> MTQAKAKHADVPVNLYRPNAPFIGKVISNEPLVKEGGIGIVQHIKFDLTGGNLKYIEGQSIGIIPPGVDKNGKPEKLRLYSIASTRHGDDVDDKTISLCVRQLEYKHPESGETVYGVCSTYLTHIEPGSEVKITGPVGKEMLLPDDPEANVIMLATGTGIAPMRTYLWRMFKDAERAANPEYQFKGFSWLVFGVPTTPNILYKEELEEIQQKYPDNFRLTYAISREQKNPQGGRMYIQDRVAEHADQLWQLIKNQKTHTYICGLRGMEEGID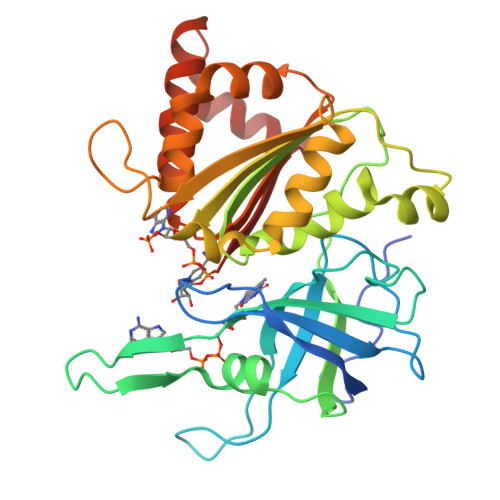AALSAAAAKEGVTWSDYQKDLKKAGRWHVETY>WNSRYSYNQLKNKDSLIMFLVEIFRSLFVSNCIDKNIDNVLLSIEEMFIDHYYNPQHSRLKYLIDDVGIFFTKLPITKAFHTYNKKYRITKRLYAPPTFNEVRHILNLAQILSLEEGLDLLTFDANETLYPDGHDFNDEVLASYISCLLKKMNIAIVTAASYNNDAEKYQKRLENLLKYFSKHNIKDGSYKNFYVMGGESNYLFKCNEEATLYSVPENEWRHYKKFVDYDTVQEILNISEKCLEKVIKDFGLCAQIQRKEKSIGLVPNKIPSLNIKNEQKNYMIKYEVLEEAVIRIKKEIIKNKITAPYCAFNGGQDLWVDVGNKAEGLLILQKLLKIQKKKCCHIGDQFLHSGNDFPTRFCSLTLWVSNPQETKACLKSIMHL[2x];>[2x]QWNSRYSYNQLKNKDSLIMFLVEIFRSLFVSNCIDKNIDNVLLSIEEMFIDHYYNPQHSRLKYLIDDVGIFFTKLPITKAFHTYNKKYRITKRLYAPPTFNEVRHILNLAQILSLEEGLDLLTFDANETLYPDGHDFNDEVLASYISCLLKKMNIAIVTAASYNNDAEKYQKRLENLLKYFSKHNIKDGSYKNFYVMGGESNYLFKCNEEATLYSVPENEWRHYKKFVDYDTVQEILNISEKCLEKVIKDFGLCAQIQRKEKSIGLVPNKIPSLNIKNEQKNYMIKYEVLEEAVIRIKKEIIKNKITAPYCAFNGGQDLWVDVGNKAEGLLILQKLLKIQKKKCCHIGDQFLHSGNDFPTRFCSLTLWVSNPQETKACLKSIMHL;> SDMKKNIVQWNSRYSYNQLKNKDSLIMFLVEIFRSLFVSNCIDKNIDNVLLSIEEMFIDHYYNPQHSRLKYLIDDVGIFFTKLPITKAFHTYNKKYRITKRLYAPPTFNEVRHILNLAQILSLEEGLDLLTFDANETLYPDGHDFNDEVLASYISCLLKKMNIAIVTAASYNNDAEKYQKRLENLLKYFSKHNIKDGSYKNFYVMGGESNYLFKCNEEATLYSVPENEWRHYKKFVDYDTVQEILNISEKCLEKVIKDFGLCAQIQRKEKSIGLVPNKIPSLNIKNEQKNYMIKYEVLEEAVIRIKKEIIKNKITAPYCAFNGGQDLWVDVGNKAEGLLILQKLLKIQKKKCCHIGDQFLHSGNDFPTRFCSLTLWVSNPQETKACLKSIMHLN;>[2x]QWNSRYSYNQLKNKDSLIMFLVEIFRSLFVSNCIDKNIDNVLLSIEEMFIDHYYNPQHSRLKYLIDDVGIFFTKLPITKAFHTYNKKYRITKRLYAPPTFNEVRHILNLAQILSLEEGLDLLTFDANETLYPDGHDFNDEVLASYISCLLKKMNIAIVTAASYNNDAEKYQKRLENLLKYFSKHNIKDGSYKNFYVMGGESNYLFKCNEEATLYSVPENEWRHYKKFVDYDTVQEILNISEKCLEKVIKDFGLCAQIQRKEKSIGLVPNKIPSLNIKNEQKNYMIKYEVLEEAVIRIKKEIIKNKITAPYCAFNGGQDLWVDVGNKAEGLLILQKLLKIQKKKCCHIGDQFLHSGNDFPTRFCSLTLWVSNPQETKACLKSIMHLN;> FVQWNSRYSYNQLKNKDSLIMFLVEIFRSLFVSNCIDKNIDNVLLSIEEMFIDHYYNPQHSRLKYLIDDVGIFFTKLPITKAFHTYNKKYRITKRLYAPPTFNEVRHILNLAQILSLEEGLDLLTFDANETLYPDGHDFNDEVLASYISCLLKKMNIAIVTAASYNNDAEKYQKRLENLLKYFSKHNIKDGSYKNFYVMGGESNYLFKCNEEATLYSVPENEWRHYKKFVDYDTVQEILNISEKCLEKVIKDFGLCAQIQRKEKSIGLVPNKIPSLNIKNEQKNYMIKYEVLEEAVIRIKKEIIKNKITAPYCAFNGGQDLWVDVGNKAEGLLILQKLLKIQKKKCCHIGDQFLHSGNDFPTRFCSLTLWVSNPQETKACLKSIMHLN

Maintaining the optimal nucleotide balance required for normal cell proliferation is controlled by 5′-nucleotidases amongst other processes. These enzymes catalyze the dephosphorylation of ribo- and deoxyribonucleoside monophosphates to their corresponding nucleosides, and also exhibit, in certain cases phosphotransferase activity. All structures adopt a tetrameric assembly displaying a cross-like shape, in agreement with the quaternary solution structure. Each subunit consists of four domains: an “N-Terminal Regulatory Domain” (NTRD, M1 to K59), an “OD” (D60 to T143), a HAD-like Catalytic Domain (CD, F144 to K270 and K371 to Q444) and a C2 cap domain13 (K271 to N370).

The crystal structures confirm that the IMP-Mg2+ substrate is mainly coordinated by conserved residues from the four HAD motifs, and by W365, which is situated on β-strand I. The base moiety of the nucleotide is stabilized by a π-stacking interaction with W365 and by three hydrogen bonds with A205 (Motif II), S207 and D367. Hydroxyl groups 2′ and 3′ of the sugar moiety form hydrogen bonds with D363 and D178, respectively, whereas the phosphate moiety of the nucleotide forms hydrogen bonds with D170 (Motif I), T204 and A205 (Motif II), K371 (Motif III), and N401 (Motif IV). Mg2+ is coordinated by the phosphate moiety, side chains of D170 (Motif I), D394 and Q395 (Motif IV), and the main chain carbonyl of D/N172. After IMP-Mg2+ or Mg2+ binding (PfISN1D172N-IMP, PfISN1WT-Mg2+), helix α8 restructures into a loop and orients the E173 side chain to accommodate the substrate. Concurrently, side chains of D178 and D394 flip into the catalytic pocket to coordinate the substrate while the breakage of the salt bridge between E173 and H398 induces a complete reorganization of the segment between D394 and F407 engendering α-helix D402-F407. Concomitantly, the four subunits bend even more than in the PfISN1-ATP conformation to adopt the most closed form observed. In this latter conformation, we do not observe the NTRDs as seen in PfISN1-Apo and PfISN1-ATP structures. Indeed, the four NTRDs are relocated at interfaces 2 beneath SegmentD394-F407. Despite adding ATP prior to crystallization, ATP molecules are not observed in PfISN1D172N-IMP structure. As concerns the IMP-binding stoichiometry, we observed that in the PfISN1D172N-IMP structure, each subunit binds one IMP-Mg2+, a feature also observed in the PfISN1D172N-ΔN30-IMP structure.>ADLQVRDIMVPRSQMISIKATQTPREFLPAVIDAAHSRYPVIGESHDDVLGVLLAKDLLPLILKADGDSDDVKKLLRPATFVPESKRLNVLLREFRANHNHMAIVIDEYGGVAGLVTIEDVLEQIVGDIEDEHD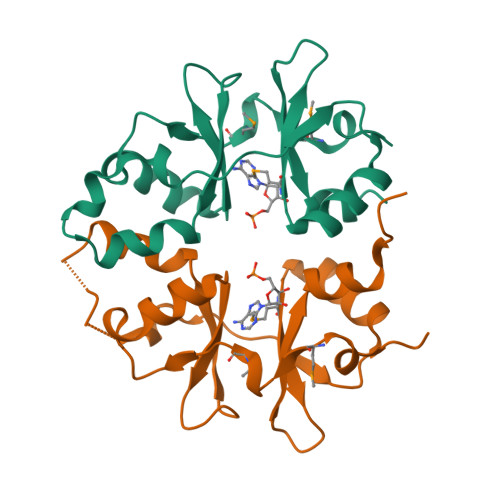VE[2x]> VQRGYGNPIEASSYGLDLDCGAPGTPEAHVCFDPCQNYTLLDEPFRSTENSAGSQGCDKNMSGWYRFVGEGGVRMSETCVQVHRCQTDAPMWLNGTHPALGDGITNHTACAHWSGNCCFWKTEVLVKACPGGYHVYRLEGTPWCNLRYCTDPSHHHHHHHH

Glycoprotein 2 (GP2) and uromodulin (UMOD) filaments protect against gastrointestinal and urinary tract infections by acting as decoys for bacterial fimbrial lectin FimH. By combining AlphaFold2 predictions with X-ray crystallography and cryo-EM, we show that these proteins contain a bipartite decoy module whose new fold presents the high-mannose glycan recognized by FimH. The structure rationalizes UMOD mutations associated with kidney diseases and visualizes a key epitope implicated in cast nephropathy.

The electron density maps reveal that the GP2 branch is a protein module (henceforth referred to as ‘decoy module’) that consists of a β-hairpin stabilized by a disulfide bond (Cx48-Cy59), packed against a globular ‘D10C’ domain with a new fold including two 310 helices, nine β-strands (βA–βI) and five intermolecular disulfides (C163-C8157, C285-C9172, C3107-C6145, C4113-C10177, C5138-C7146). Interestingly, although the GP2 branch also binds FimHL, its D10C domain cannot be glycosylated at the position corresponding to UMOD N275 (R165). In agreement with these considerations, introduction of an N65A mutation in the decoy module of GP2 impairs its interaction with FimHL and mass spectrometric analysis of the glycans attached to N65 detects the HexNAc2Hex5 oligomannose structure, indicating that UMOD and GP2 exploit a common molecular strategy to counteract bacterial adhesion. Because of 60% sequence identity to UMOD, the crystal structure of the latter immediately explains the effect of many substitutions affecting invariant positions. Remarkably, most of these mutations cluster within two structurally important regions of the decoy module, the β-hairpin/D10C domain groove and the disulfide bond-rich region at the opposite end of D10C.>[3x]NLYQFKNMIKCTVPSRSWWDFADYGCYCGRGGSGTPVD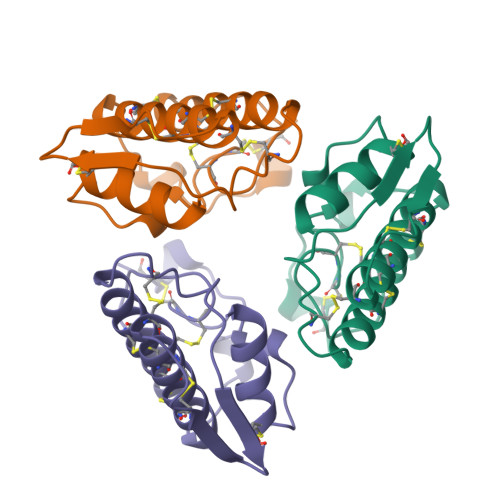DLDRCCQVHDNCYNEAEKISGCWPYFKTYSYECSQGTLTCKGDNNACAASVCDCDRLAAICFAGAPYNDNNYNIDLKARCQ>MGNAQERPSETIDRERMRLVETLQADSGLLLDALLARGVLTGPEYEALDALPDAERRVRRLLLLVQ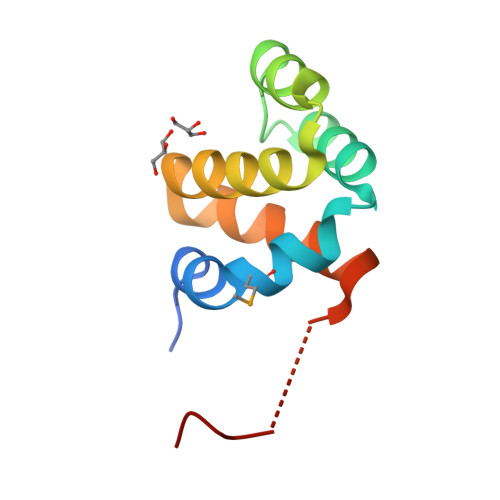GKGEAACQELLRCAQRTAGAPDPAWDWQH[2x]> MSDDNSHSSDTISNKKGFFSLLLSQLFHGEPKNRDELLALIRDSGQNDLIDEDTRDMLEGVMDIADQRVRDIMIPRSQMITLKRNQTLDECLDVIIESAHSRFPVISEDKDHIEGILMAKDLLPFMRSDAEAFSMDKVLRQAVVVPESKRVDRMLKEFRSQRYHMAIVIDEFGGVSGLVTIEDILELIVGEIEDEYDEEDDIDFRQLSRHTWTVRALASIEDFNEAFGTHFSDEEV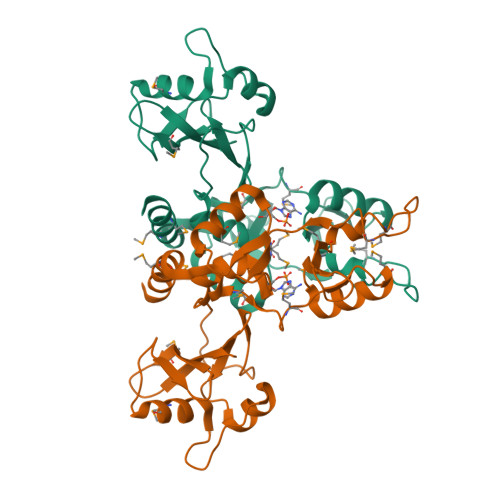DTIGGLVMQAFGHLPARGETIDIDGYQFKVAMADSRRIIQVHVKIPDDSPQPKLDE>MRGSHHHHHHGSMTDTYLHETLVFDNKLSYIDNQRDTDGPAILLLPGWCHDHRVYKYLIQELDADFRVIVPNWRGHGLSPSEVPDFGYQEQVKDALEILDQLGVETFLPVSHSHGGWVLVELLEQAGPERAPRGIIMDWLMWAPKPDFAKSLTLLKDPERWREGTHGLFDVWLDGHDEKRVRHHLLEEMADYGYDCWGRSGRVIEDAYGRNGSPMQMMANLTKTRPIRHIFSQPTEPEYEKINSDFAEQHPWFSYAKLGGPTAFPAIDVPDRAAVHIREFA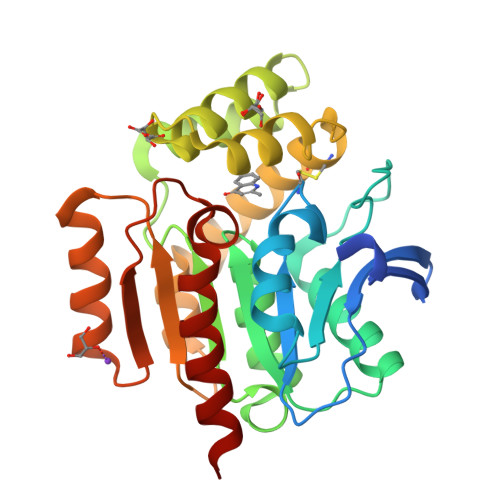TAIRQGQ[2x]>[2x]GPKFPRVKNWELGSITYDTLCAQSQQDGPCTPRRCLGSLVLPRKLQTRPSPGPPPAEQLLSQARDFINQYYSSIKRSGSQAHEERLQEVEAEVA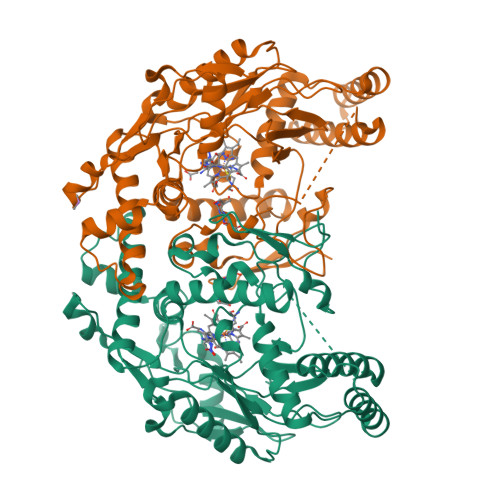STGTYHLRESELVFGAKQAWRNAPRCVGRIQWGKLQVFDARDCSSAQEMFTYICNHIKYATNRGNLRSAITVFPQRAPGRGDFRIWNSQLVRYAGYRQQDGSVRGDPANVEITELCIQHGWTPGNGRFDVLPLLLQAPDEAPELFVLPPELVLEVPLEHPTLEWFAALGLRWYALPAVSNMLLEIGGLEFSAAPFSGWYMSTEIGTRDLCDPHRYNILEDVAVCMDLDTRTTSSLWKDKAAVEINLAVLHSFQLAKVTIVDHHAATVSFMKHLDNEQKARGGCPADWAWIVPPISGSLTPVFHQEMVNYILSPAFRYQPDPW>[3x]QIDITKLQHVGVLVNSPKGMK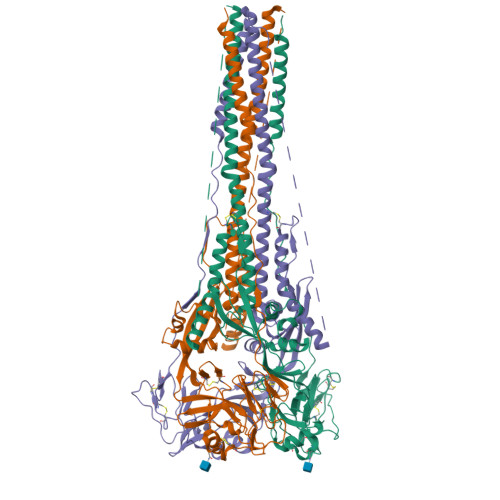ISQNFETRYLILSLIPKIEDSNSCGDQQIKQYKRLLDRLIIPLYDGLRLQKDVIVSNQESNENTDPSTKRFFGGVIGTIALGVATSAQITAAVALVEAKQARSDIEKLKEAIRDTNKAVQSVQSSIGNLIVAIKSVQDYVNKEIVPSIARLGCEAAGLQLGIALTQHYSELTNIFGDNIGSLQEKGIKLQGIASLYRTNITEIFTTSTVDKYDIYDLLFTESIKVRVIDVDLNDYSITLQVRLPLLTRLLNTQIYRVDSISYNIQNREWYIPLPSHIMTKGAFLGGADVKECIEAFSSYICPSDPGFVLNHEMESCLSGNISQCPRTVVKSDIVPRYAFVNGGVVANCITTTCTCNGIGNRINQPPDQGVKIITHKECNTIGINGMLFNTNKEGTLAFYTPNDITLNNSVALDPIDISIELNKAKSDLEESKEWIRRSNQKLDSIGNWHQSSTTGGPLVPRGSHHHHHH methyl 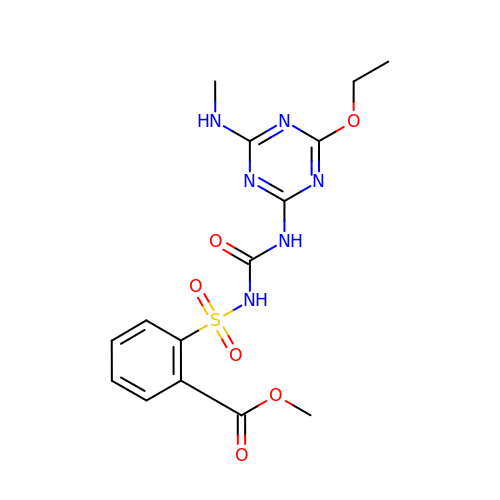2-[[4-ethoxy-6-(methylamino)-1,3,5-triazin-2-yl]carbamoylsulfamoyl]benzoate | C15 H18 N6 O6 S | ZINJLDJMHCUBIP-UHFFFAOYSA-N5-AMINO-1-(5-O-PHOSPHONO-BETA-D-RIBOFURANOSYL)-1H-IMIDAZOLE-4-CARBOXYLIC ACID | C9 H14 N3 O9 P | 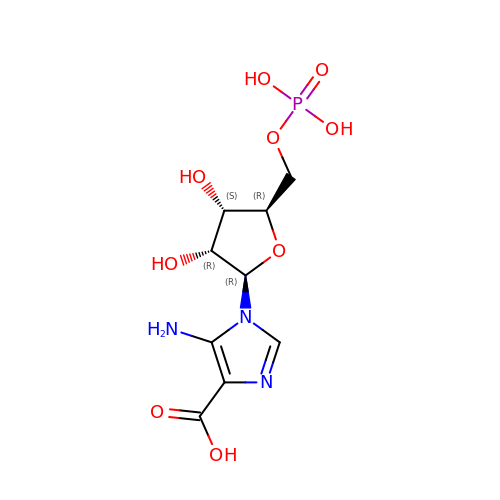XFVULMDJZXYMSG-ZIYNGMLESA-N We have focused our work on the iron(II)/α-KetoAcid-dependent Oxygenases (αKAOs), a mechanistically diverse superfamily of enzymes that use dioxygen as the oxidant to catalyze several reactions via C-H bond activation, mostly hydroxylation. These enzymes operate with three substrates, dioxygen, α-ketoglutarate (α-KG) and a primary substrate. One of these, KDO1, catalyzes the formation of (3S)-3-hydroxy-L-lysine, while five others, KDO2 to KDO6, promote the formation of (4R)-4-hydroxy-L-lysine. We based our analysis on the structures that we solved by X-ray crystallography of two of the regiodivergent αKAOs active towards L-lysine, namely KDO1 from Catenulispora acidiphila, that catalyzes the C-3 hydroxylation, and KDO5, from Flavobacterium sp., that catalyzes the C-4 hydroxylation.

In all four molecules of each of the KDO5 structures, an iron ion is present in the active site chelated by two His (176 and 312) and one Glu (178). In α-KG bound structure, α-KG is best defined for monomer A. The carboxylate moieties of the co-substrate form salt bridges with Arg338 and 334 (2.9 Å; 2.8 Å and 3.1 Å); the α-ketoacid moiety binds the iron as bidentate; the terminal carboxylate interacts by H-bond with Tyr193 (3.0 Å).

>MKSQSIMSVERSAETSLTLEIPTSPLIIKITQQERNILSNVGNLLVKAFGNYENPDYIASLHLHAFQLLPERITRILSQFGSDFSAEQYGAIVFQGLIEVDQDDLGPTPPNWQGADYGKLNKYGFICSLLHGAVPSKPVQYYAQRKGGGLLHAVIPDEKMAATQTGSGSKTDLFVHTEDAFLSNQADFLSFLYLRNEERVPSTLYSIRSHGKMNPVMKKLFEPIYQCPKDANYNDEDVANSGPTASVLYGNRELPFIRFDAAEQIFNENAGQTSEALGNLMDFWDEAKTLINSDYIPNSGDLIFVNNHLCAHGRSAFIAGQRIENGEIIKCERRQMLRMMSKTSLIHIRSVTRTDDPYFIMEEHLGKIFDLD[4x]2-[({4-[(2-amino-4-oxo-4,7-dihydro-3H-pyrrolo[2,3-d]pyrimidin-5-yl)methyl]benzene-1-carbonyl}amino)methyl]benzoic 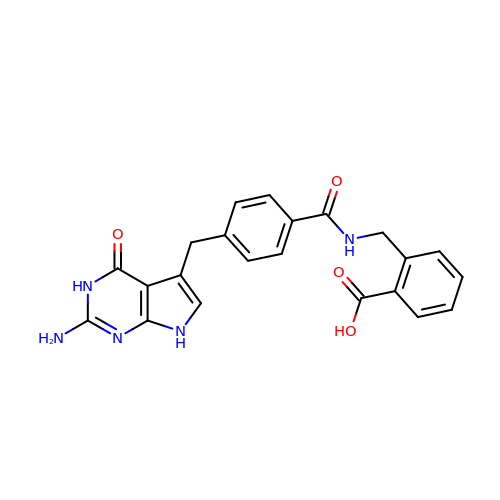acid | C22 H19 N5 O4 | BBGUOTHUKQSSGG-UHFFFAOYSA-N> MVYPQPKVLTPSRKDVLVVTPWLAPIVWEGTFNIDILNEQFRLQNTTIGLTVFAIKKYVAFLKLFLETAEKHFMVGHRVHYYVFTDQPAAVPRVTLGTGRQLSVLEVGAYKRWQDVSMRRMEMISDFSERRFLSEVDYLVSVDVDM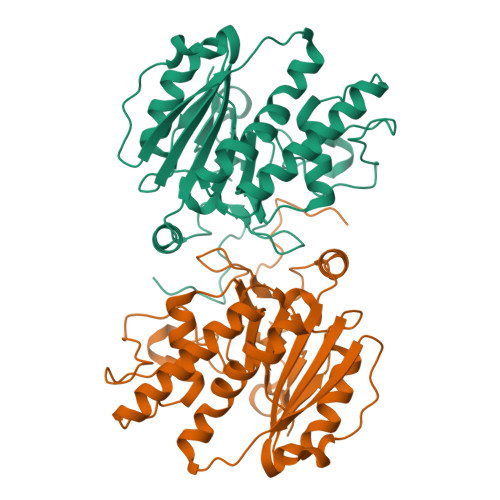EFRDHVGVEILTPLFGTLHPSFYGSSREAFTYERRPQSQAYIPKDEGDFYYMGAFFGGSVQEVQRLTRACHQAMMVDQANGIEAVWHDESHLNKYLLRHKPTKVLSPEYLWDQQLLGWPAVLRKLRFTAVPKNHQAVRNPE> MDRQGFVPAAYVKKLDSGTGKELVLALYDYQ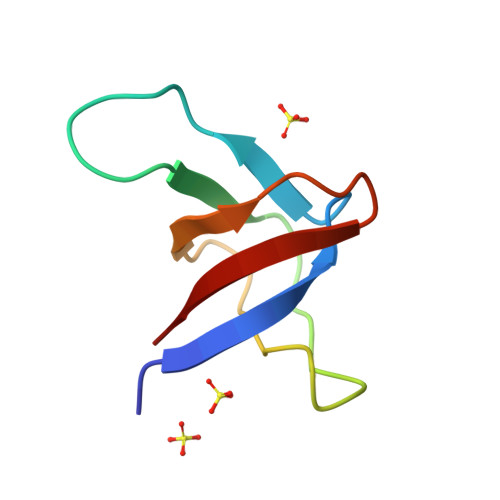EKSPREVTMKKGDILTLLNSTNKDWWKVEVN> HHHHHHLESTSLYKKAGFMGVVEEAHNVKVIGSGEATIVLGHGFGTDQSVWKHLVPHLV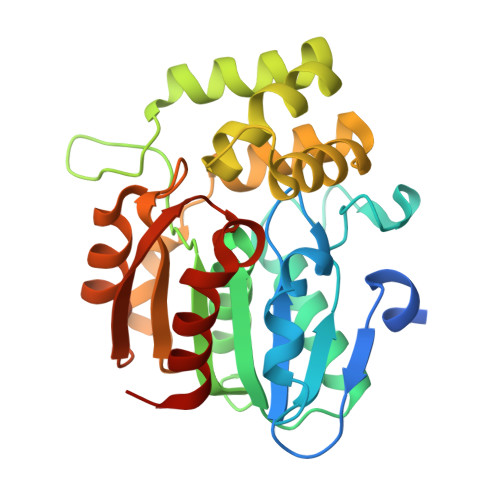DDYRVVLYDNMGAGTTNPDYFDFDRYSNLEGYSFDLIAILEDLKIESCIFVGHSVSAMIGVLASLNRPDLFSKIVMISASPRYVNDVDYQGGFEQEDLNQLFEAIRSNYKAWCLGFAPLAVGGDMDSIAVQEFSRTLFNMRPDIALSVGQTIFQSDMRQILPFVTVPCHILQSVKDLAVPVVVSEYLHANLGCESVVEVIPSDGHLPQLSSPDSVIPVILRHIRNDIAM>MSLQSAQYLRQAEVLKADMTDSKLGPAEVWTSRQALQDLYQKMLVTDLEYALDKKVEQDLWNHAFKNQITTLQGQAKNRANPNRSEVQANLSLFLEAASGFYTQLLQELCTVFNVDLPCRVKSSQLGIISNKQTHTSAIVKPQSSSCSYICQHCLVHLGDIARYRNQTSQAESYYRHAAQLVPSNGQPYNQLAILASSKGDHLTTIFYYCRSIAVKFPFPAASTNLQKALSKALESRDEVKTKWGVSDFIKAFIKFHGHVYLSKSLEKLSPLREKLEEQFKELLFQKAFNSQQLVHVTVINLFQLHHLRDFSNETEQHTYSQDEQLCWTQLLALFMSFLGILCKCPLQNESQ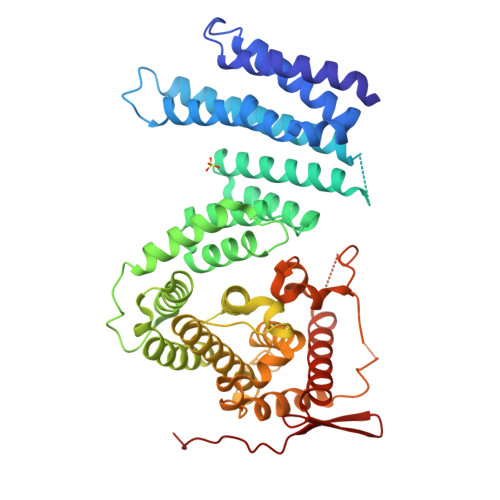EESYNAYPLPAVKVSMDWLRLRPRVFQEAVVDERQYIWPWLISLLNSFHPHEEDLSSISATPLPEEFELQGFLALRPSFRNLDFSKGHQGITGDKEGQQRRIRQQRLISIGKWIADNQPRLIQCENEVGKLLFITEIPELILEDP[2x]> MHHHHHHLPNITILATGGTIAGGGDSATKSNYTVGKVGVENLVNAVPQLKDIANVKGEQVVNIGSQDMNDNVWLTLAKKINTDCDKTDGFVITHGTDTMEETAYFLDLTVKCDKPVVMVGAMRPSTSMSADGPFNLYNAVVTAADKASANRGVLVVMNDTVLDGRDVTMTNTTDVATFKSVNYGPLGYIHNGKIDYQRTPARKHTSDTPFDVSKLNELPKVGIVYNYANASDLPAKALVDAGYDGIVSAGVGNGNLYKSVFDTLATAAKTGTAVVRSSRVPTGATTQDAEVDDAKYGFVASGTLNPQKARVLLQL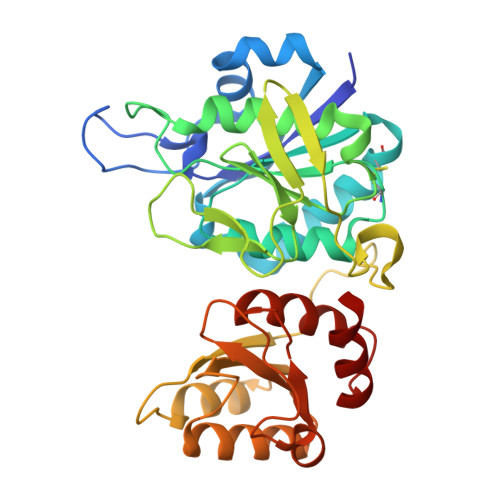ALTQTKDPQQIQQIFNQY> MENTENSVDSKSIKNLEPKIIHGSESMDSGISLDNSYKMDYPEMGLCIIINNKNFHKSTGMTSRSGTDVDAANLRETFRNLKYEVRNKNDLTREEIVELMRDVSKEDHSKRSSFVCVLLSHGEEGIIFGTNGPVDLKKIFNFFRGDRCRSLTGKPKLFIIQACRGTELDCGIETDSGVDDDMACHKIPVEADFLYAYSTAPGY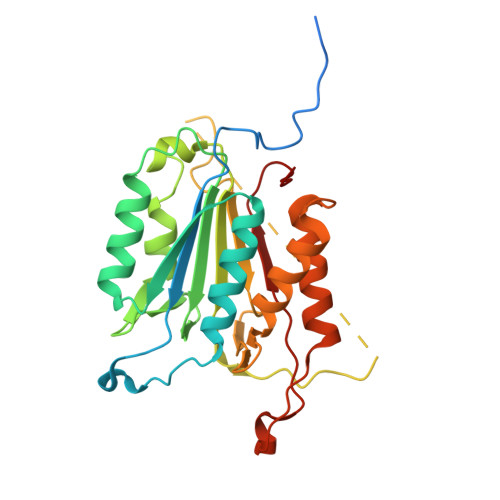YSWRNSKDGSWFIQSLCAMLKQYADKLEFMHILTRVNRKVATEFESFSFDATFHAKKQIPCIVSMLTKELYFYH>MFSKLAHLQRFAVLSRGVHSSVASATSVATKKTVQG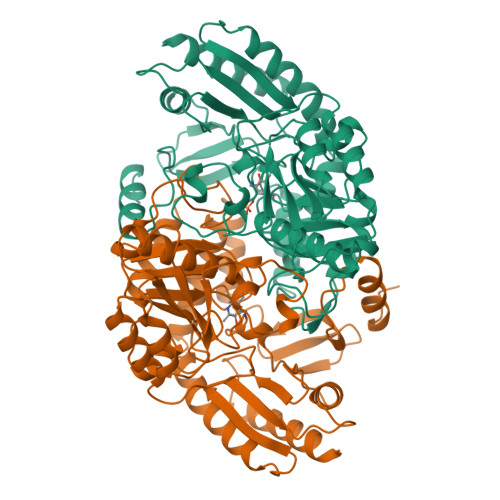PPTSDDIFEREYKYGAHNYHPLPVALERGKGIYLWDVEGRKYFDFLSSISAVNQGHCHPKIVNALKSQVDKLTLTSRAFYNNVLGEYEEYITKLFNYHKVLPMNTGVEAGETACKLARKWGYTVKGIQKYKAKIVFAAGNFWGRTLSAISSSTDPTSYDGFGPFMPGFDIIPYNDLPALERALQDPNVAAFMVEPIQGEAGVVVPDPGYLMGVRELCTRHQVLFIADEIQTGLARTGRWLAVDYENVRPDIVLLGKALSGGLYPVSAVLCDDDIMLTIKPGEHGSTYGGNPLGCRVAIAALEVLEEENLAENADKLGIILRNELMKLPSDVVTAVRGKGLLNAIVIKETKDWDAWKVCLRLRDNGLLAKPTHGDIIRFAPPLVIKEDELRESIEIINKTILSF[3x]> GSMNQATQIIPFTTSGSLVDYVDRKVIVVLRDGKKLIGILRSFDQFANLMLQYTIERIYVDDMYGDIDRGVYIVRGENVVLLGELD;> MLFYSFFKTLIDTEVTVELKNDMSIRGILKSVDQFLNVKLENISVVDASKYPHMAAVKDLFIRGSVVRYVHMSSAYVDTILLADACRRDLANNKRQ;> GSMESAQAVAEPLDLVRLSLDEIVYVKLRGDRELNGRLHAYDEHLNMVLGDAEEIVTIFDDEETDKDKALKTIRKHYEMLFVRGDSVILIAPPRN;> MLPLTLLNATQGRPILVELKNGETFNGHLENCDNYMNLTLREVIRTMPDGDKFFRLPECYIRGNNIKYLRIQDEVLSQVAKQQAQQRENRGSRFRGRGQRGRGNYGHTAPNRRGRGRGGHMWSHPQFEK;> MSMTILPLELIDKCIGSNLWVIMKSEREFAGTLVGFDDYVNIVLKDVTEYDTVTGVTEKHSEMLLNGNGMCMLIPGGKPE;> GSMDSSPNEFLNKVIGKKVLIRLSSGVDYKGILSCLDGYMNLALERTEEYVNGKKTNVYGDAFIRGNNVLYVSALDD;> MSSLQKRPGPGNSSQPTERPRKESILDLSRYQDQRIQATFTGGRQ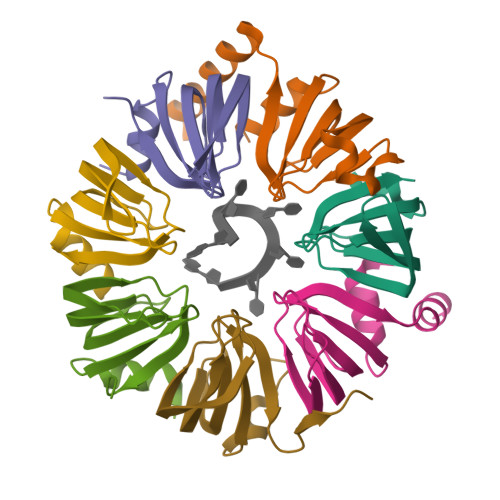ITGILKGFDQLMNLVLDDVEEQLRNPEDGKLTGAIRKLGLVVVRGTTLVLIAPMDGSEEIPNPFVQAE> MAVPFVEDWDLVQTLGE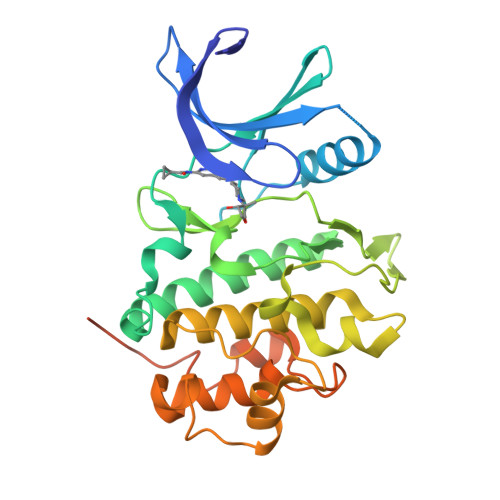GAYGEVQLAVNRVTEEAVAVKIVDMKRAVDCPENIKKEICILKMLNHENVIKFYGHRREGNIQYLFMELASGGSLFDRIEPDIGMPEPDAQRFFHQLMAGVVYLHGIGITHRDIKPHNLLLDERDNLKIADYSLATVFRYNNRERLLNKMCGTLPYVAPELLKRREFHAEPVDVWSCGIVLTAMLAGELPWDQPSDSCQEYSDWKEKKTYLNPWKKIDSAPLALLHKILVENPSARITIPDIKKDRWYNKPLKKGAKRPRVTSGGVSESPSGHHHHHHHH> MNLFWPSETKKQNEIPGGDYTPGNSPSVQKGYQFLNRDIFKSCPRIMERQFGECLHNRTHLIKDLISSGNVGLGPIEIVHMSYLNKHEKEEFGEYFYVTGIEVSGPAMPVEFLEVLKSSKRISKNISNNIILTYCCFNFFSNLDIRIRYDADDTFQTTAIDCNKETTDLTMTEKMWEETFASSVIRAIITNTNPELKPPGLVECPFYVGKDTISSCKKIIELLCRFLPRSLNCGWDSTKSMQATIVNNYLMYSLKSFIAITPSLVDFTIDYLKGLTKKDPI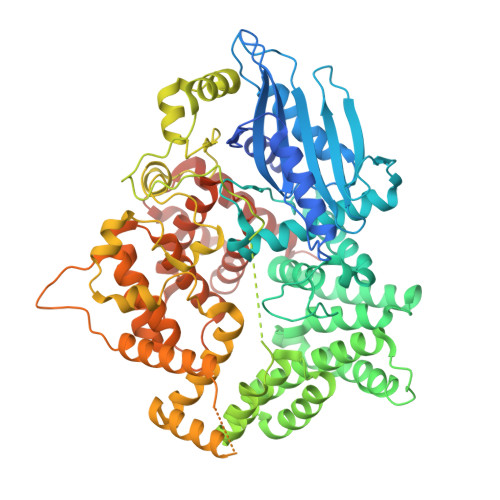HDIYYKTAMITILDHIETKELDMITILNETLDPLLSLLNDLPPRDADSARLMNCMSDLLNIQTNFLLNRGDYELALGVSNTSTELALDSFESWYNLARCHIKKEEYEKALFAINSMPRLRKNDGHLETMYSRFLTSNYYKKPLNGTREHYDLTAMEFTNLSGTLRNWKEDELKRQIFGRIAMINEKKIGYTKEIWDDIAIKLGPICGPQSVNLINYVSPQEVKNIKNINLIARNTIGKQLGWFSGKIYGLLMEIVNKIGWNGLLNIRTEAFMMETEFYQASNNIIDENGHIPMESRKKRFCEGWLDDLFLDLYQDLKLSKISLSNKDEKHSGLEWELLGLIMLRTWHWEDAVACLRTSIVARFDPVSCQQLLKIYLQPPKNIQEVTLLDTDTIISLLIKKISYDCRYYNYCQIFNLQLLEKLCNELGTHILRNKILLQPSIGDEIMVMIDAMLAWIADLDHTVQPGTENLYFQGHHHHHH>GPGSMSGAGNLRSNRRREMDYMRLCNSTRKVYPSDTVAEFWVEFKGPEGTPYEDGTW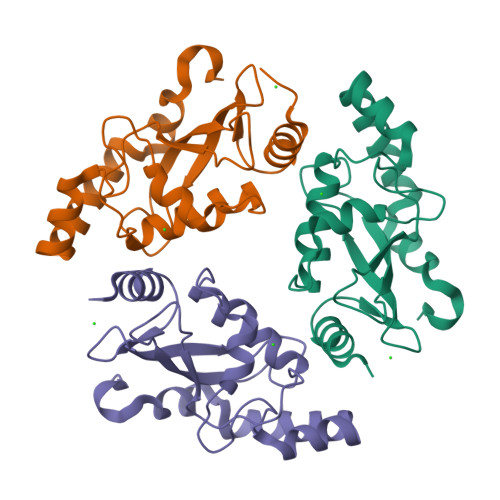MLHVQLPSDYPFKSPSIGFCNRILHPNVDERSGSVCLDVINQTWTPMYQLENIFDVFLPQLLRYPNPSDPLNVQAAHLLHADRVGFDALLREHVSTHATPQKALESIPEAYRPH[3x]>MAEESRGQRGSGYGLGLSTRTQVTGYQFLARRTAMALTRWRVRMEIEPGRRQTLAVVASVSAALVICLGALLWSFISPSGQLNESPIIADRDSGALYVRVGDRLYPALNLASARLITGRPDNPHLVRSSQIATMPRGPLVGIPGAPSSFSPKSPPASSWLVCDTVATSSSIGSLQGVTVTVIDGTPDLTGHRQILSGSDAVVLRYGGDAWVIREGRRSRIEPTNRAVLLPLGLTPEQVSQARPMSRALFDALPVGPELLVPEVPNAGGPATFPGAPGPIGTVIVTPQISGPQQYSLVLGDGVQTLPPLVAQILQNAGSAGNTKPLTVEPSTLAKMPVVNRLDLSAYPDNPLEVVDIREHPSTCWWWERTAGENRARVRVVSGPTIPVAATEMNKVVSLVKADTSGRQADQVYFGPDHANFVAVTGNNPGAQTSESLWWVTDAGARFGVEDSKEARDALGLTLTPSLAPWVALRLLPQGPTLSRADALVEHDTLPMDMTPAELVVPK[6x];>[6x]MKRGFARPTPEKPPVIKPENIVLSTPLSIPPPEGKPWWLIVVGVVVVGLLGGMVAMVFASGSHVFGGIGSIFPLFMMVGIMMMMFRGMGGGQQQMSRPKLDAMRAQFMLMLDMLRETAQESADSMDANYRWFHPAPNTLAAAVGSPRMWERKPDGKDLNFGVVRVGVGMTRPEVTWGEPQNMPTDIELEPVTGKALQEFGRYQSVVYNLPKMVSLLVEPWYALVGEREQVLGLMRAIICQLAFSHGPDHVQMIVVSSDLDQWDWVKWLPHFGDSRRHDAAGNARMVYTSVREFAAEQAELFAGRGSFTPRHASSSAQTPTPHTVIIADVDDPQWEYVISAEGVDGVTFFDLTGSSMWTDIPERKLQFDKTGVIEALPRDRDTWMVIDDKAWFFALTDQVSIAEAEEFAQKLAQWRLAEAYEEIGQRVAHIGARDILSYYGIDDPGNIDFDSLWASRTDTMGRSRLRAPFGNRSDNGELLFLDMKSLDEGGDGPHGVMSGTTGSGKSTLVRTVIESLMLSHPPEELQFVLADLKGGSAVKPFAGVPHVSRIITDLEEDQALMERFLDALWGEIARRKAICDSAGVDDAKEYNSVRARMRARGQDMAPLPMLVVVIDEFYEWFRIMPTAVDVLDSIGRQGRAYWIHLMMASQTIESRAEKLMENMGYRLVLKARTAGAAQAAGVPNAVNLPAQAGLGYFRKSLEDIIRFQAEFLWRDYFQPGVSIDGEEAPALVHSIDYIRPQLFTNSFTPLEVSVGGPDIEPVVAQPNGEVLESDDIEGGEDEDEEGVRTPKVGTVIIDQLRKIKFEPYRLWQPPLTQPVAIDDLVNRFLGRPWHKEYGSACNLVFPIGIIDRPYKHDQPPWTVDTSGPGANVLILGAGGSGKTTALQTLICSAALTHTPQQVQFYCLAYSSTALTTVSRIPHVGEVAGPTDPYGVRRTVAELLALVRERKRSFLECGIASMEMFRRRKFGGEAGPVPDDGFGDVYLVIDNYRALAEENEVLIEQVNVIINQGPSFGVHVVVTADRESELRPPVRSGFGSRIELRLAAVEDAKLVRSRFAKDVPVKPGRGMVAVNYVRLDSDPQAGLHTLVARPALGSTPDNVFECDSVVAAVSRLTSAQAPPVRRLPARFGVEQVRELASRDTRQGVGAGGIAWAISELDLAPVYLNFAENSHLMVTGRRECGRTTTLATIMSEIGRLYAPGASSAPPPAPGRPSAQVWLVDPRRQLLTALGSDYVERFAYNLDGVVAMMGELAAALAGREPPPGLSAEELLSRSWWSGPEIFLIVDDIQQLPPGFDSPLHKAVPFVNRAADVGLHVIVTRTFGGWSSAGSDPMLRALHQANAPLLVMDADPDEGFIRGKMKGGPLPRGRGLLMAEDTGVFVQVAATEVRR;>MTAVADAPQADIEGVASPQAVVVGVMAGEGVQIGVLLDANAPVSVMTDPLLKVVNSRLRELGEAPLEATGRGRWALCLVDGAPLRATQSLTEQDVYDGDRLWIRFIADTERRSQVIEHISTAVASDLSKRFARIDPIVAVQVGASMVATGVVLATGVLGWWRWHHNTWLTTIYTAVIGVLVLAVAMLLLMRAKTDADRRVADIMLMSAIMPVTVAAAAAPPGPVGSPQAVLGFGVLTVAAALALRFTGRRLGIYTTIVIIGALTMLAALARMVAATSAVTLLSSLLLICVVAYHAAPALSRRLAGIRLPVFPSATSRWVFEARPDLPTTVVVSGGSAPVLEGPSSVRDVLLQAERARSFLSGLLTGLGVMVVVCMTSLCDPHTGQRWLPLILAGFTSGFLLLRGRSYVDRWQSITLAGTAVIIAAAVCVRYALELSSPLAVSIVAAILVLLPAAGMAAAAHVPHTIYSPLFRKFVEWIEYLCLMPIFPLALWLMNVYAAIRYR[12x]

Specialized protein transport systems—known as type VII secretion systems (T7SSs)—are central to the virulence of this pathogen, and are also crucial for nutrient and metabolite transport across the mycobacterial cell envelope. Mycobacterium tuberculosis encodes five homologous, but functionally distinct, T7SSs that are designated ESX-1 to ESX-5. These systems translocate a number of effector proteins across the unique and impermeable diderm cell envelope. Here we reconstituted the ESX-5 T7SS of M. tuberculosis H37Rv in M. smegmatis to obtain a structural view of the entire T7SS membrane complex from this human pathogen.

To further investigate the effect of MycP5 on the entire structure, we analysed MycP5-free M. tuberculosis ESX-5 complexes from the same preparation. These assemblies contained the same EccB5:EccC5:EccD5:EccE5 stoichiometry as the fully assembled complexes. Following 3D reconstruction, we obtained two MycP5-free M. tuberculosis ESX-5 maps that displayed resolution estimates of about 4.5 and about 6.7 Å. The differences were most notable on the periplasmic side, on which the six EccB5 copies showed high flexibility and did not form a stable triangular scaffold in the absence of MycP5. This shows that MycP5 enables the trimerization of the EccB5 dimers in the periplasm. In contrast to the periplasmic domain, the cytosolic and membrane regions of the MycP5-free maps were more similar to those of the MycP5-containing particles. However, the MycP5-free particles displayed an increased heterogeneity that affected the entire complex, which resulted in a slight waving of the membrane region and an increased angle variation between individual protomers. Complexes without MycP5 show disruption of the EccB5 periplasmic assembly and increased flexibility, which highlights the importance of MycP5 for complex integrity. Our MycP5-free M. tuberculosis ESX-5 maps are reminiscent of the hexameric, low-resolution negative-stain structure of ESX-5 from Mycobacterium xenopi, in which the periplasm was similarly disorganized in the absence of MycP55.>MMKVTPIALLLAGVLASPLCAAGLDAQLTLVDGSTDDVRVNLTLTNTGDKPIRLLKWQLPGSDDAPLFLVERDGQPVSYEGALIKRAAPTDKDFQLLKAGQSLTVQAEVSGLYDMSAQGQYSIRYQLPARRKRPRAKQAQASESNAITLWVEGVNDERVQAKVAAAEPQAVAGSVSFSGRCTNTQKSDLLTALDAASGISNNASSYLAVDKPDGQRYRSWFGAYSSARWDQAETNFSKIKDAIDNKPLTFDCSCKQSYFAYVYPDQPYKVYLCKSFWTAPVTGSDSRAGTIVHALSHFNVVAGTDDLGYGQANARNLAKTDPVKALNNADNHEYF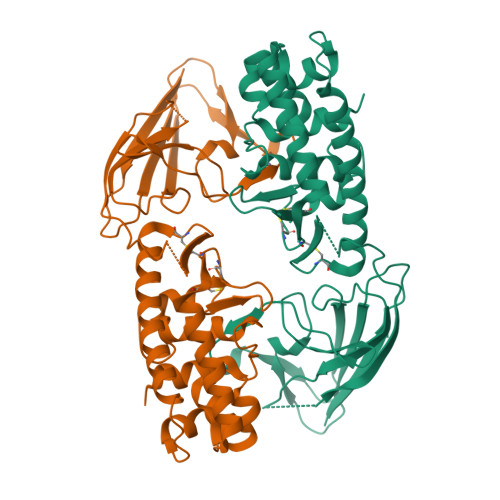AENTPSEN[2x]> MTTACPARTSSLMDDLLGLLRIRIKRGVNLAVRDISSSDPYVVVKMGSQKLKTRVINKDVNPEWNEDLTLSVTDSNLTVLLTVYDHDMFSKDDKMGDAEFEIKPYIEALRMQLGGLPSGTIVTTVKPSRRNCLAEESRVTWVDGKLVQDLVL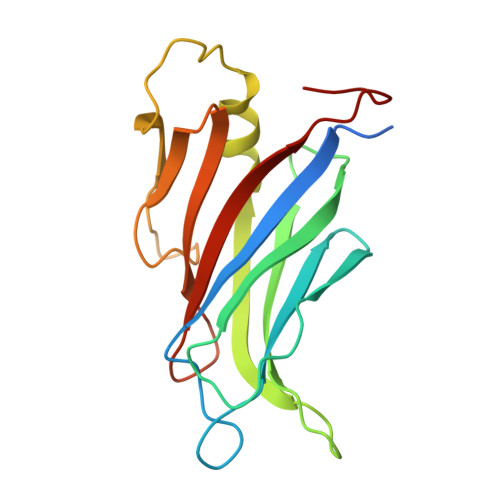RLRHVECGEVEAQLQWIDLPGSSGL>[2x]GSAMADIGAEIKQGIREVILCKDQDGKIGLRLKSVDNGIFVQLVQANSPASLVGLRFGDQVLQINGENCAGWSSDKAHKVLKQAFG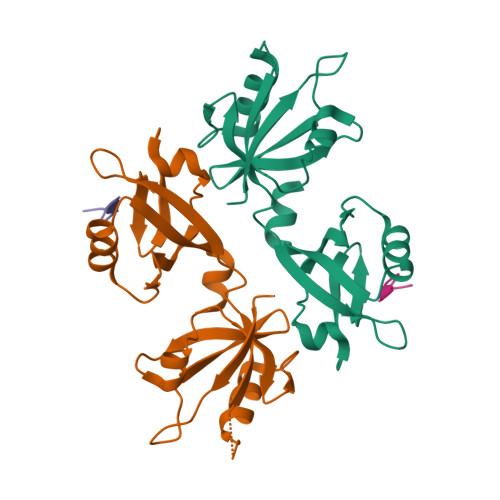EKITMTIRDRPFERTVTMHKDSSGHVGFIFKSGKITSIVKDSSAARNGLLTDHHICEINGQNVIGLKDAQIADILSTAGTVVTITIMPAFIFEHIIKRMAPSIMKSLMDHTIPEV;>[2x]APTNEFYA> MAAAAGGPCVRSSRELWTILLGRSALRELSQIEAELNKHWRRLLEGLSYYKPPSPSSAEKVKANKDVASPLKELGLRISKFLGLDEEQSVQLLQCYLQEDYRGTRDSVKTVLQDERQSQALILKIADYYYEERTCILRCVLHLLTYFQDERHPYRVEYADCVDKLEKELVSKYRQQFEELYKTEAPTWETHGNLMTERQVSRWFVQCLREQSMLLEIIFLYYAYFEMAPSDLLVLTKMFKEQGFGSRQTNRHLVDETMDPFVDRIGYFSALILVEGMDIESLHKCALDDRRELHQFAQDGLICQDMDCLMLTFGDIPHHAPVLLAWALLRHTLNPEETSSVVRKIGGTAIQLNVFQYLTRLLQSLASGGNDCTTSTACMCVYGLLSFVLTSLELHTLGNQQDIIDTACEVLADPSLPELFWGTEPTSGLGIILDSVCGMFPHLLSPLLQLLRALVSGKSTAKKVYSFLDKMSFYNELYKHKPHDVISHEDGTLWRRQTPKLLYPLGGQTNLRIPQGTVGQVMLDDRAYLVRWEYSYSSWTLFTCEIEMLLHVVSTADVIQHCQRVKPIIDLVHKVISTDLSIADCLLPITSRIYMLLQRLTTVISPPVDVIASCVNCLTVLAARNPAKVWTDLRHTGFLPFVAHPVSSLSQMISAEGMNAGGYGNLLMNSEQPQGEYGVTIAFLRLITTLVKGQLGSTQSQGLVPCVMFVLKEMLPSYHKWRYNSHGVREQIGCLILELIHAILNLCHETDLHSSHTPSLQFLCICSLAYTEAGQTVINIMGIGVDTIDMVMAAQPRSDGAEGQGQGQLLIKTVKLAFSVTNNVIRLKPPSNVVSPLEQALSQHGAHGNNLIAVLAKYIYHKHDPALPRLAIQLLKRLATVAPMSVYACLGNDAAAIRDAFLTRLQSKIEDMRIKVMILEFLTVAVETQPGLIELFLNLEVKDGSDGSKEFSLGMWSCLHAVLELIDSQQQDRYWCPPLLHRAAIAFLHALWQDRRDSAMLVLRTKPKFWENLTSPLFGTLSPPSETSEPSILETCALIMKIICLEIYYVVKGSLDQS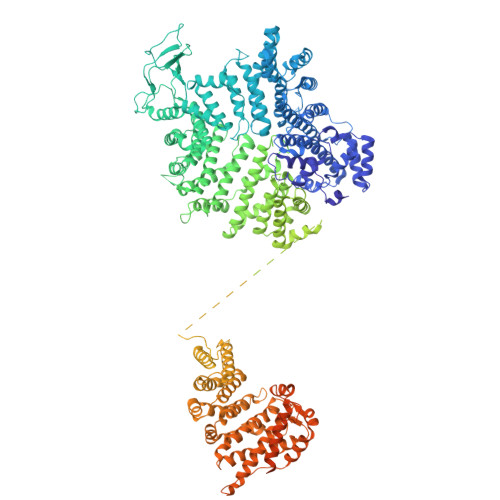LKDTLKKFSIEKRFAYWSGYVKSLAVHVAETEGSSCTSLLEYQMLVSAWRMLLIIATTHADIMHLTDSVVRRQLFLDVLDGTKALLLVPASVNCLRLGSMKCTLLLILLRQWKRELGSVDEILGPLTEILEGVLQADQQLMEKTKAKVFSAFITVLQMKEMKVSDIPQYSQLVLNVCETLQEEVIALFDQTRHSLALGSATEDKDSMETDDCSRSRHRDQRDGVCVLGLHLAKELCEVDEDGDSWLQVTRRLPILPTLLTTLEVSLRMKQNLHFTEATLHLLLTLARTQQGATAVAGAGITQSICLPLLSVYQLSTNGTAQTPSASRKSLDAPSWPGVYRLSMSLMEQLLKTLRYNFLPEALDFVGVHQERTLQCLNAVRTVQSLACLEEADHTVGFILQLSNFMKEWHFHLPQLMRDIQVNLGYLCQACTSLLHSRKMLQHYLQNKNGDGLPSAVAQRVQRPPSAASAAPSSSKQPAADTEASEQQALHTVQYGLLKILSKTLAALRHFTPDVCQILLDQSLDLAEYNFLFALSFTTPTFDSEVAPSFGTLLATVNVALNMLGELDKKKEPLTQAVGLSTQAEGTRTLKSLLMFTMENCFYLLISQAMRYLRDPAVHPRDKQRMKQELSSELSTLLSSLSRYFRRGAPSSPATGVLPSPQGKSTSLSKASPESQEPLIQLVQAFVRHMQR> AGAGAAGAUUUUUUU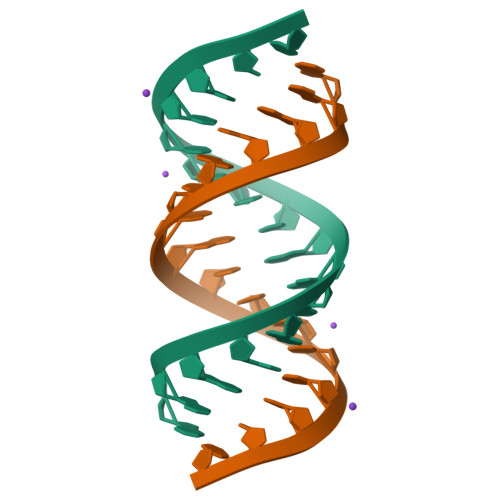U> MGRSWHYVEPKFLNKAFEVALKVQIIAGFDRGLVKWLRVHGRTLSTVQK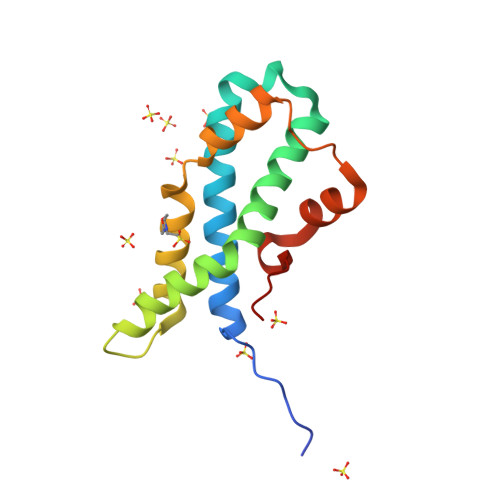KALYFVNRRYMQTHWANYMLWINKKIDALGRTPVVGDYTRLGAEIGRRIDMAYFYDFLKDKNMIPKYLPYMEEINRMRPADVPVKYMGK1-(1-methylindol-3-yl)ethanone | C11 H11 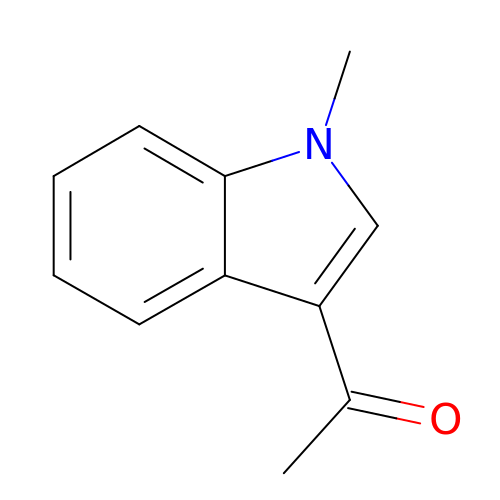N O | HYLFRICFKVJJOZ-UHFFFAOYSA-N>RGSHMSLSKKRKLESGDSGGAGAGGEGAEEENGGEQEAAPPRPRRTKSERDQLYYECYSDVSVHEEMIADQVRTEAYRLGILKNWAALRGKTVLDVGAGTGILSIFCAQAGARRVYAVEASAI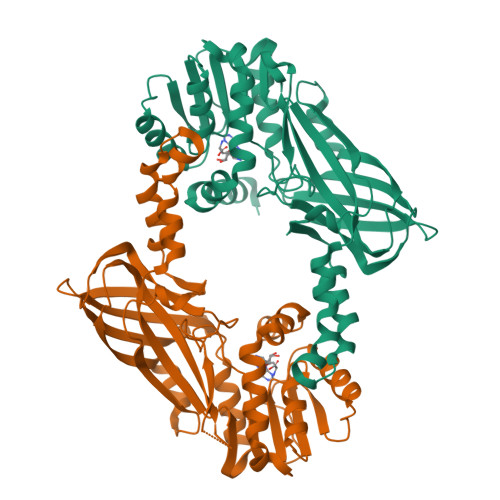WQQAREVVRLNGLEDRVHVLPGPVETVELPERVDAIVSEWMGYGLLHESMLSSVLHARTKWLKEGGLLLPASAELFVAPISDQMLEWRLGFWSQVKQHYGVDMSCMESFATRCLMGHSEIVVQDLSGEDVLARPQRFAQLELARAGLEQELEAGVGGRFRCSCYGSAPLHGFAVWFQVTFPGGDSEKPLVLSTSPLHPATHWKQALLYLNEPVPVEQDTDISGEITLLPSPDNPRRLRILLRYKVGDHEEKTKDFAMED[2x]> QIDQYAVFGNPINHSKSPFIHTLFARQTQQSMIYTAQCVPVDGFTEAAKHFFAQGGRGCNVTVPFKEEAYRFADRLTERARLAGAVNTLKKLDDGEILGDNTDGEGLVQDLLAQQVLLKGATILLIGAGGAARGVLKPLLDQQPASITVTNRTFAKAEQLAELVAAYGEVKAQAFEQLKQSYDVIINSTSASLDGELPAIDPVIFSSRSVCYDMMYGKGYTVFNQWARQHGCAQAIDGLGMLVGQAAESFMLWR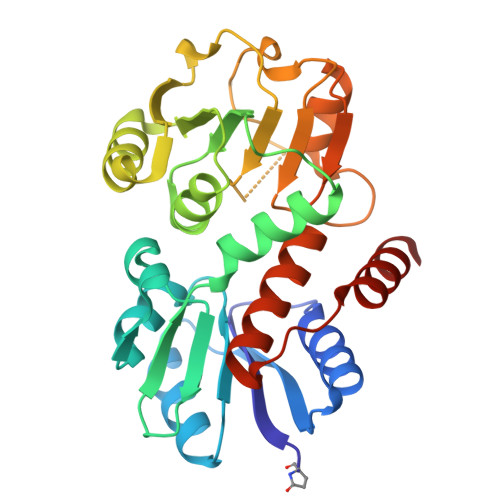GLRPGTKQILRELRKNLEGAL> GDPVKPSRGPLVTCTCESPHCKGPTCRGAWCTVVLVREEGRHPQEHRGCGNLHRELCRGRPTEFVNHYCCDSHLC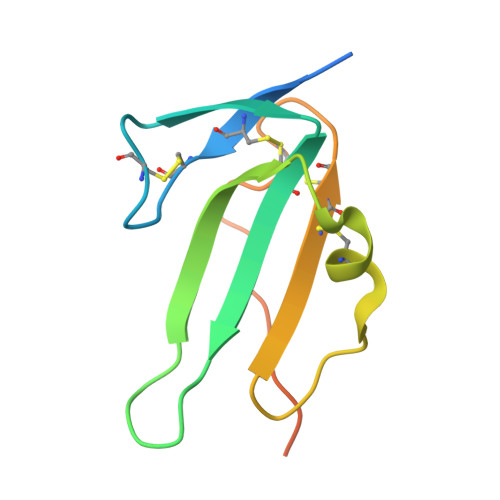NHNVSLVLEATQPPSEQPGTDGQ> MQKLLSPRTARHARLFRLAGKLADSGSPGVPKSDGERLVWVNSHVRRDKDISLSQEE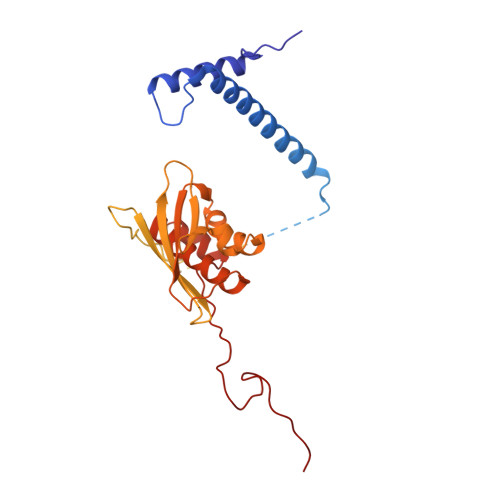ERIRELMMPLEVGENSFAANGQATHGNLFYFREYPMYPGEYVPAEHNTLSSLRDELRLDLTAQSLKEAWMRVSGGVYFQSVDEYYASVDGLDAEQIGEVLAALFPELNCYEAQALVQRTLECISRPVSAASRQLSRTITAEAVGLDNAPGHYTNFLEWMGRLTETRAFKTEHALFEFSRRKFNRDDVRVMFENYRLMSKATLLADSADSYSHFYTVLKDFAXKVAGEDSRHQIGVRIDEAEVDPETGIAVGRGCADGEKYHFTALLRENRDHNGIITVMGKPLSLVLDNKAWLMEMVLMPFDEANLDYRDFDAHIVSEGHAMPSIANEIAAFALRMAVANALVKLIPLTRIPLKKSGLLSVDRRRERGQFPGYLDGKKVKRRFAKR(3R,4S)-1-[(4-amino-5H-pyrrolo[3,2-d]pyrimidin-7-yl)methyl]-4-[(pyrazin-2-ylsulfanyl)methyl]pyrrolidin-3-ol 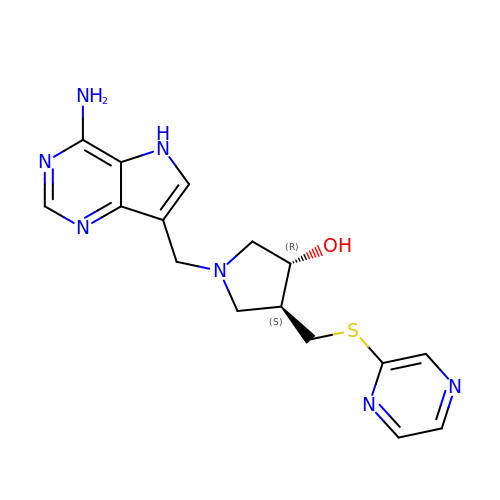| C16 H19 N7 O S | UMOBRIXOOIFSTP-NEPJUHHUSA-N> SNAMPYTWKFLGISKQLSLENGIAKLNQLLNLEVDLDIQTIRVPSDPDGGTAADEYIRYEMRLDISNLDEGTYSKFIFLGNSKMEVPMFLCYCGTDNRNEVVLQWLKAEYGVIMWPIKFEQKTMIKLADASIVHVTKENIEQITWFSSKLYFEPETQDKNLRQFSIEIPRESCEGLALGYGNTMHPYNDAIVPYIYNETGMAVERLPLTSVILAGHTKIMRESIVTSTRSLRNRVLAVVLQSIQFTSE;> SNAMSRIDDLQQDIESLLSEINSLEESREKLKAKIKDKRKNEESANPIVQEFEDLFDQFPQLNNFLFNEHPELEETDDKDISRAQADIPATPIPYEPKKRAKLENEEILPEQEWVLKTQPMVQHQMFDPGVADLLDTDILTSPSKRKRKLKIDDISTSDRSELEDYIVLENVYRMFGITFFPLVDPIDLKIKDASGEIFVDREMLGIRLEVFSERTSQFEKPHYVLLKKRIKSNSWFLFKHTIPSFIDVQGIFDDTNGGLVISHDDAYLFAKRVFLQLVEVQKRRQIFKDLEAKKIIHDLDLDLESSMVSFFVKDIKVELFVKQNEIVSCSILDDIHDFSQNNKSKWEIALLGSLDDLELKLNHSFATIFK;> MDFTSDTTNSHDTSNSHLSLEDAVGTHHAGEADVNIDGDEKQQLSLLDDDQVRALKLQEEKDALLTRRNTLLQEIQTYQNILMKENNSKTKNGDILQNDITQDFLNLISISSSNPNSAISDRKRVERINGLTNLQKELVTKYDTLPLLNMNLRLSYLRDHTYPHLQVSVQSRDRVHNDGIEVLVVNYKFCRNTMNPFEIQFKMFYKFEDSTLLKWEILRISTNVRLKAKQLLATRNFQKCLLSLYEFDKIKSKKTGIFQNLINLLKRKTRCYLMNNSDSLIVERVIREGRLTTIKLQINFIITMPGERGKPRNCFLPMSKISIALWKGGERFNQIDLDEICYGLIKEYGVKTGLKEICNVCLFPDMYAR;> SNAMSNELRLEDNYVPTSDTLVVFKQLMKLPVTVLYDLTLSWFAKFGGSFDGDIYLLTETLDLLIEKGVRRNVIVNRILYVYWPDGLNVFQLAEIDCHLMISKPEKFKWLPSKALRGDGKPYVVKLQPAKFIENLQTDLAKIYHCHVYMFKHPSLPVLITRIQLFDSNNLFLSTPNIGSINKESLYNKLDKFQGKPLISRRPYYVAFPLNSPIIFHSVDKDIYARLVLQSISRTISERETIIFKPVQKIPVKSIHNIMTLLGPSRFAESMGPWECYASANFERSPLHDYKKHQGLTGKKVMVREFDDSFLNDDENFYGKEEPEIRRLRLEKNMIKFKGSANGVMDQKYNDLKEFNEHVHNIRNGKKNEDSGEPVYISRYSSLVPIEKVGFTLKNEINSRIITIKLKFNGNDIFGGLHELCDKNLINIDKVPGWLAGENGSFSGTIMNGDFQREQVAKGGLL;> MAADRDNFLQNIENDSINNGQAMDLSPNRSSSESDSSILMNVNDIKTLRLDVAPEAKSTQSKKSLFYENSDDAEEGEIEERTNKEEGQYHHKGSKQLRFEVGKESTGKLQSHLSDGSATSGEGNVRPWEFRKVIQAEYRERLPRNYELKHWKKPSKIMIGSILRLLETNTVSALDSVFEKYEKEMNQMTHGDNNEVKRIYSKKERLLEIILTKIKKKLRQAKFPSRISERDLDIEYIYSKRQFIQNRYSQELQNNERLEAILSREQNLLEETRKLCMNLKTNNKKRLTEKLIQKDLHPVLNKAMEYTYGLESTNGFMHPDGPVTFRNDSHELNLMLNDPIKSTADVRLDKEEVLSLLPSLKEYTKKSKELKETMGQMISDSHEEEIKEVFVPHHESHQDKTEEDIH;> SNAMTDTYNSISNFIENELTALLSSDDYLMDDLAGELPNEVCRLLKAQVIEKRKDAMSRGKQDLLSKEIYDNESELRASQSQQIMELVGDIPKYSLGSELRNRVEGEPQSTSIERLIEDVLKLPQMEVADEEEVEVENDLKVLSEYSNLRKDLILKCQALQIGESKLSDILSQTNSINSLTTSIKEASEDDDISEYFATYNGKLVVALEEMKLLLEEAVKTFGNSPEKREKIKKILSELKK;>SNAMSLILDDIILSLTNANERTPPQALKTTLSLLYEKSKQYGLSSPQLQALVRLLCETSIIDTVTKVYIVENCFLPDGYLTKELLLEIINHLGTPTVFSRYRIQTPPVLQSALCKWLVHVYFLFPVHSEREHNISSSIWLHLWQFSFLQKWITPLVIWQATTPVDVKPWKLSIIKRCAMHPGYRDAPGSATLILQRFQCLVGASSQITESIITINCNRKTLKSHRNLKLDAHFLSILKRILSRAHPANFPADTVQNTIDMYLSEIHQLGADSIYPLRLQSLPEYVPSDSTVSLWDVTSLEQLAQNWPQLHIPNDVDYMMKPSLNSNVLLPRKVMSRDSLKHLYSSIILIKNSRDESSSPYEWCIWQLKRCFAHQIETPQEVIPIIISVSSMDNKLSSRIIQTFCNLKYLKLDELTLKKVCGGILPLWKPELISGTREFFVKFMASIFMWSTRDGHDNNCTFSETCFYVLQMITNWVLDDKLIALGLTLLHDMQSLLTLDKIFNNATSNRFSTMAFISSLDILTQLSKQTKSDYAIQYLIVGPDIMNKVFSSDDPLLLSAACRYLVATKNKLMQYPSTNKFVRMQNQYIMDLTNYLYRNKVLSSKSLFGVSPDFFKQILENLYIPTADFKNAKFFTITGIPALSYICIIILRRLETAENTKIKFTSGIINEETFNNFFRVHHDEIGQHGWIKGVNNIHDLRVKILMHLSNTANPYRD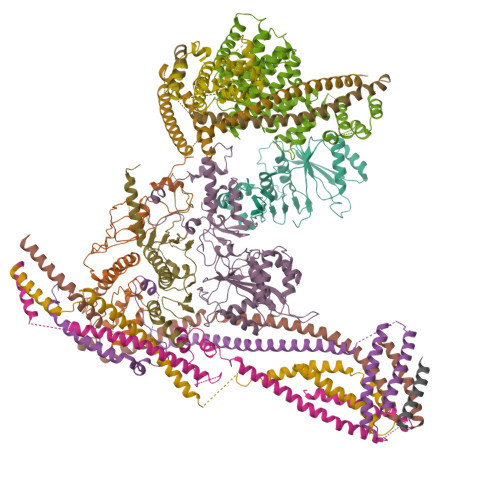IAAFLFTYLKSLSKYSVQNSXXXXXXXXXXXXXXXXXXXXXXXXXXXXXXXXXXXXX[2x];> MDRDTKLAFRLRGSHSRRTDDIDDDVIVFKTPNAVYREENSPIQSPVQPILSSPKLANSFEFPITTNNVNAQDRHEHGYQPLDAEDYPMIDSENKSLISESPQNVRNDEDLTTRYNFDDIPIRQLSSSITSVTTIDVLSSLFINLFENDLIPQALKDFNKSDDDQFRKLLYKLDLRLFQTISDQMTRDLKDILDINVSNNELCYQLKQVLARKEDLNQQIISVRNEIQELKAGKDWHDLQNEQAKLNDKVKLNKRLNDLTSTLLGKYEGDRKIMSQDSEDDSIRDDSNILDIAHFVDLMDPYNGLLKKINKINENLSNELQPSLHHHHHH;> MNSEQLLHNYVSDSLLTTLISFQEFKQQLQSYTSDEQQLQHWYELLQARDARVTSELEARIKQFFITLRSRLLRFLESEQLSHSLSLETLIDALYKINDLLQQRLQILDDAIQEKTSELAEFENMVRSPSAGDNAIPGLLQIIQSYINLLEEN> MTDHARGTLPEIRRGRIYRDVYHKRVDEEPVDRTADLERARLGDDGLDFQDDAAQARAFAQGVFLLEIPEWLDLSAGDRFARQFFQGTGVEPYGKYRDLSSEHFGDELLGYHS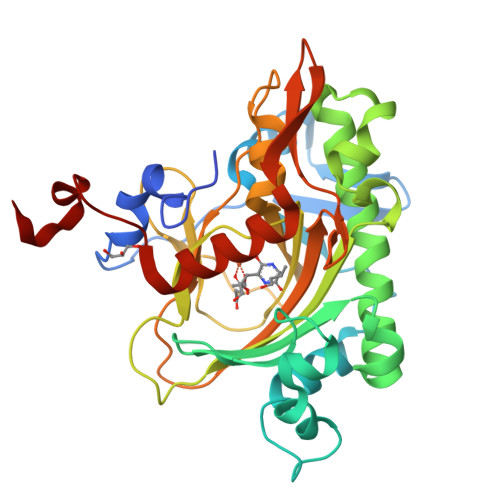RVDQLEQFLLERRFWGEVYPSEIATLGEHLTLLSHRVLRSVLASAGIPEEDWHRASGGCSETNGSYHLTFNHYRSAHQDIGLSSHKDDGFITVLRTTAQGLEVNRDDVWEKVPVDPACFVVNFGLSMEILTSACVTPLSAIMHRVSHQNFDRSSFGHFSSSRCLPGADDGIYRYLPSAGLERVCGSRELIEENAHEIYMGTEGQGLEHHHHHHHH> DVSFRLSGADPSSYGMFIKDLRNALPHTEKVYNIPLLLPSVSGAGRYLLMHLFNYDGNTITVAVDVTNVYIMGYLALTTSYFFNEPAADLASQYVFRSARRKITLPYSGNYERLQIAAGKPREKIPIGLPALDTA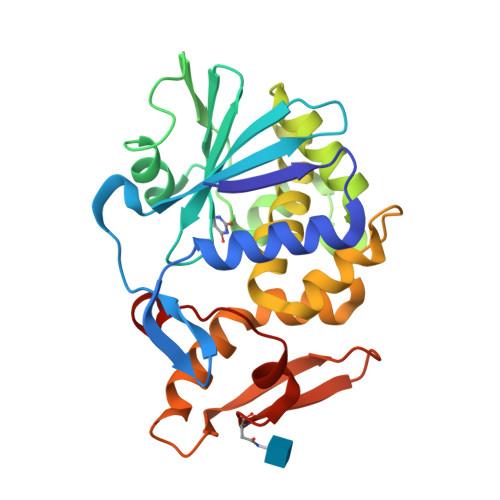ISTLLHYDSTAAAGALLVLIQTTAEAARFKYIEQQIQERAYRDEVPSSATISLENSWSGLSKQIQLAQGNNGVFRTPTVLVDSKGNRVQITNVTSNVVTSNIQLLLNTKNI> MLRLNLRFLSFLLCISQSVELQAAPSVPTFLTENGLTYCTHASGFSFNPQTADAGTSMNVVTEQIYNKLFDIKNHSATLTPMLAQSYSISADGKEILLNLRHGVKFHQTPWFTPTRDFNA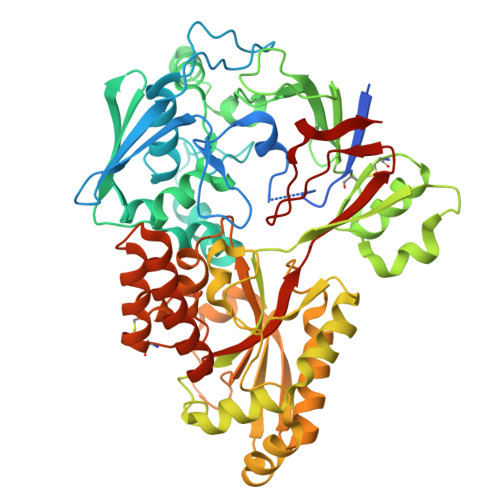EDVVFSINRVLGHNTYLPTLAEANVTYSNPQYRVFHEQARKVRFPYFDSIKLNEKIKSVTALSPYQVKIELFAPDSSILSHLASQYAIIFSQEYAYQLSADDNLAQLDTHPVGTGPYQVKDYVYNQYVRLVRNENYWKKEAKIEHIIVDLSTDRSGRLVKFFNNECQIASYPEVSQIGLLKNDDKHYYMQSTDGMNLAYLAFNFDKPLMRDHEIRAAISQSLNRARIIHSIYHNTATVANNIIPEVSWASTVNTPEFEFDYHPKIAKNKLADKNLLLNLWVINEEQVYNPAPFKMAEMIKWDLAQAGVKVKVRAVTRPFLTAQLRNQSENYDLILSGWLAGNLDPDGFMRPILSCGTKNELTNLSNWCNEEFDQFMDRAITTSHLSSRAKAYNEAQELVLRELPIIPIANVKRILVANSRVKGVKMTPFGSLDFSTLYFIQEKH> SMSDTRLDVATLANAVQLAARAPSLHNTQPWRLIAEDGELKLFLDPSRVVRSTDRSSREAVMSCGVLLDHLRVALAAAGWDTEVQRFPNPNDRDHLATLSFRPLQFVTEGHRKRADAILARRTDRLPMSAYVDWDAFETLLRARLGDGPVHMDTLGEDVREEVAEAAALTESLRLYDAAYHSELAWWTTPFATEDGIPQTALISAEESERVAVSRDFPVAPHSSRRPALNNDAATIVVLSTDGYSREDALDAGEGLSKVLLECTMSGLATCPVTHVTELHTSRDIIGRLIVRDACPQVLVRI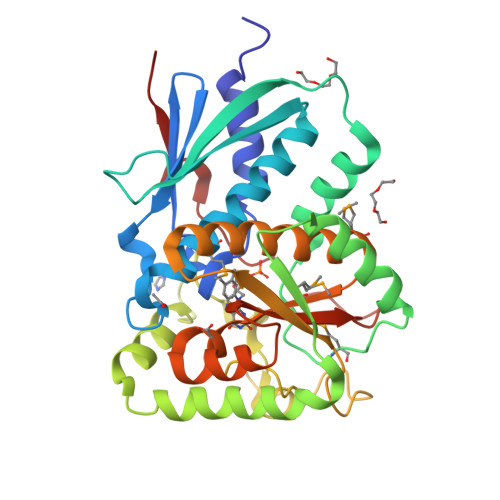GLAPALDEVPPPTPRRPVDAFLEVRPRS> MRGSHHHHHHGSLYKELVELYKRLEKTTLKTLKTKFVSDFLKSVEKPELLEVIPYLILGKVFPDWDERELGIGEKLLIKAVSMATGINSEEIENSVRDTGDLGESIALALNKRKQKSFFSQPLTIERVYNTLVKIAEASGAGSQDRKLKYLANLFMDASPDEGKYLARTVLGIMRTGVAEGLLRDALADAFKVRVELVERAYMLTSDFGFVAKVAKLEGDEGLAKVKIQVGKPIKPMLAQMAANVREALVEMGGEAEFEIKYDGARVQVHKNGNKVLIYSRRLENVTKSIPEVVERVKEALK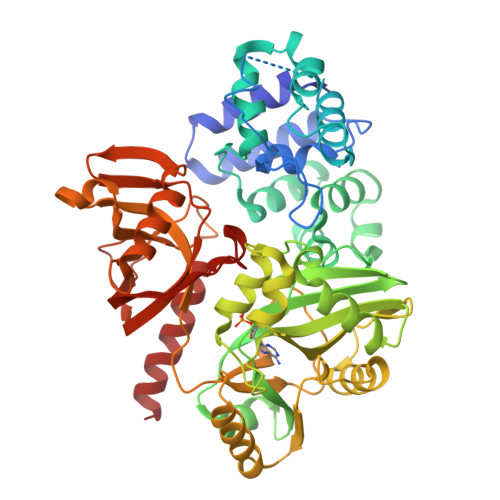PEKVIVEGELVAVEETGRPRPFQYVLRRFRRKYNIEEMIEKIPLELNLFDILYVDGQNMIDTPFMERRKVLESVVNSNEWIKSAENLITKSPEEAEAFYHKALDLGHEGLMAKRLDSTYEPGNRGKKWLKIKPTMENLDLVVLGAEWGEGRRSGVLSSFLLGAYDPVKGDFVPVGKVGSGFTDEDLVEFTKMLKPLIKKEHGKEVELEPKVVIEVAYQEIQKSPKYESGFALRFPRYIALREDKGPEDADTVQRLAELYQFQERLKGGR> HHHHHHLANTSAHDFSYLKFVYNATDTSLEGSYDYIVIGGGTSGCPLAATLSEKYKVLLLERGTIATEYPNTLTADGFAYNLQQQDDGKTPVERFVSEDGIDNVRARILGGTTIINAGVYARANISFYSQTGIEWDLDLVNKTYEWVEDAIVVKPNNQSWQSVIGEGFLEAGILPDNGFSLDHEAGTRLTGSTFDNNGTRHAADELLNKGDPNNLLVAVQASVEKILFSSNTSNLSAIGVIYTDSDGNSHQAFVRGNGEVIVSAGTIGTPQLLLLSGVGPESYLSSLNITVVQPNPYVGQFVYDNPRNFINILPPNPIEASVVTVLGIRSDYYQVSASSLPFSTPPFSLFPTTSYPLPNSTFAHIVSQVPGPLSHG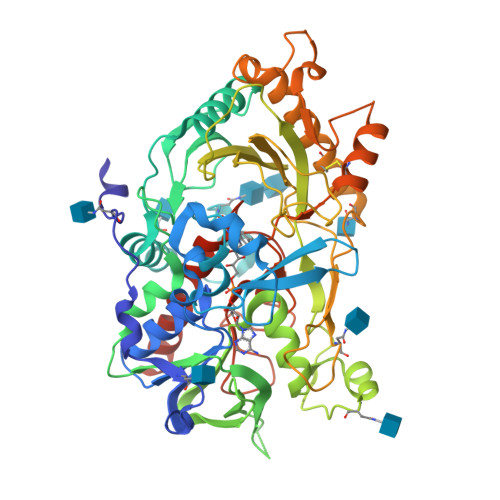SVTLNSSSDVRIAPNIKFNYYSNSTDLANCVSGMKKLGDLLRTKALEPYKARDVLGIDGFNYLGVPLPENQTDDASFETFCLDNVASYWHYHGGSLVGKVLDDSFRVMGIKALRVVDASTFPYEPNSHPQGFYLMLGRYVGLQILQERSIRLEAIHNIQESM> ILSKLATNEEHGENSPYFDGWKAYDSDPFHPLKNPNGVIQMGLAENQLCLDLIEDWIKRNPKGSICSEGIKSFKAIANFQDYHGLPEFRKAIAKFMEKTRGGRVRFDPERVVMAGGATGANETIIFCLADPGDAFLVPSPYYPAFNRDLRWRTGVQLIPIHCESSNNFKITSKAVKEAYENAQKSNIKVKGLILTNPSNPL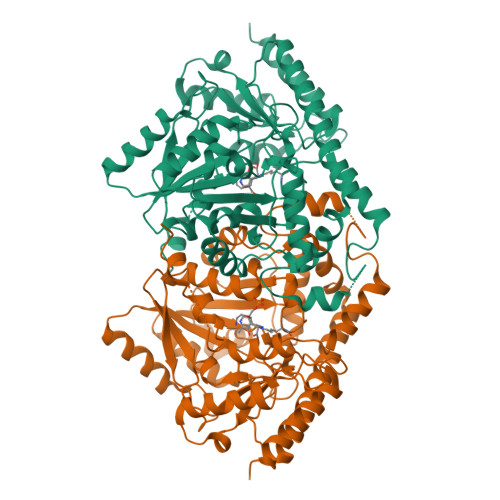GTTLDKDTLKSVLSFTNQHNIHLVCDEIYAATVFDTPQFVSIAEILDEQEMTYCNKDLVHIVYSLSKDMGLPGFRVGIIYSFNDDVVNCARKMSSFGLVSTQTQYFLAAMLSDEKFVDNFLRESAMRLGKRHKHFTNGLEVVGIKCLKNNAGLFCWMDLRPLLRESTFDSEMSLWRVIINDVKLNVSPGSSFECQEPGWFRVCFANMDDGTVDIALARIRRFVGVEK> AASERKALQTEMARIKKWLTFSLGKQVGNKFFLTNGEIMTFEKVKALCVKFQASVATPRNAAENGAIQNLIKEEAFLGITDEKTEGQFVDLTGNRL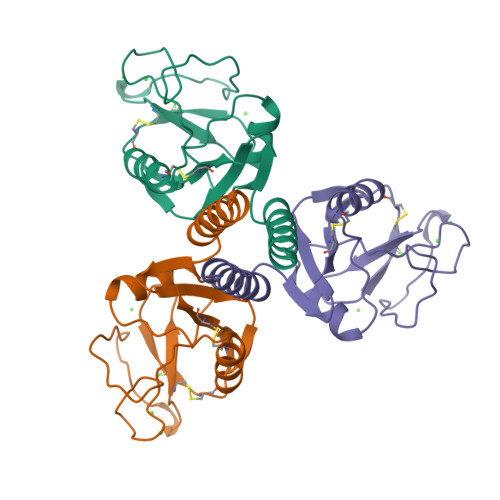TYTNWNEGEPNNAGSDEDCVLLLKNGQWNDVPCSTSHLAVCEFPI> PLGSQYFLKVLIPSYAAGSIIGKGGQTIVQLQKETGATIKLSKSKDFYPGTTERVCLIQGTIEALNAVHGFIAEKIREMPQNVAKTEPVSILQPQTTVNP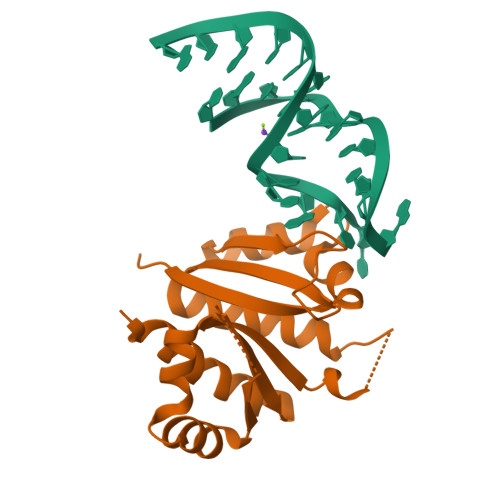DRANQVKIIVPNSTAGLIIGKGGATVKAIMEQSGAWVQLSQKPDGINLQNRVVTVSGEPEQNRKAVELIIQKIQEDPQ> GMDPNEAVREFAKEIDVSYVKI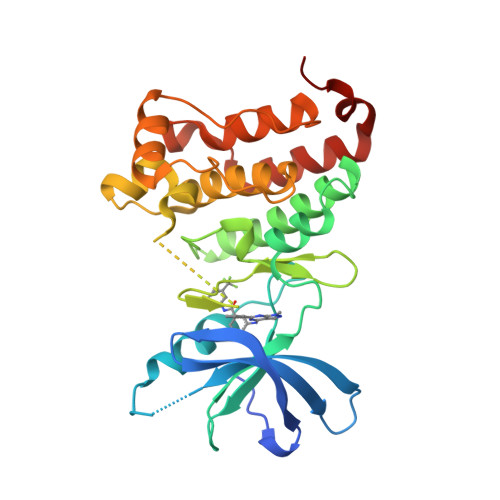EEVIGAGEFGEVCRGRLKAPGKKESCVAIKTLKGGYTERQRREFLSEASIMGQFEHPNIIRLEGVVTNSMPVMILTEFMENGALDSFLRLNDGQFTVIQLVGMLRGIASGMRYLAEMSYVHRDLAARNILVNSNLVCKVSDFGLSRFLEENSSDPTETSSLGGKIPIRWTAPEAIAFRKFTSASDVWSYGIVMWEVMSFGERPYWDMSNQDVINAIEQDYRLPPPPDCPTSLHQLMLDCWQKDRNARPRFPQIVSALDKMIRNPASLKIVARENG>MNVASRVVVNADRVKGTINRNIYGHFSEHLGRCIYEGLWVGEDSPIPNTNGIRNDVLEALKQMKIPVLHWPGGCFADEYHWKDGVGPREKRKRMVNTHWGGVIENNHFGTHEFMMLCELLGCEPYISGNVGSGTVQEMSEWVEYITFDGESPMANWRRENGREKPWRIKYWGVGNENWGCGGNMRAEYYADLYRQFQTYLRNYGDNKLHKIACGAWTADYHWTEVLMKQAAPFMHGLSLHYYTVPGPWEKKGPATGFTTDEWWVTLKKALFMDELVTKHSAIMDVYDPDKRIDLIVDEWGTWYDVEPGTNPGFLYQQNSIRDALVAGATLHIFHRHCDRVRMANIAQLVNVMQSVILTEGERMLLTPTYHVFNMFKVHQDAELLDTWESVERTGPEGELPKVSVSASRAADGKIHISL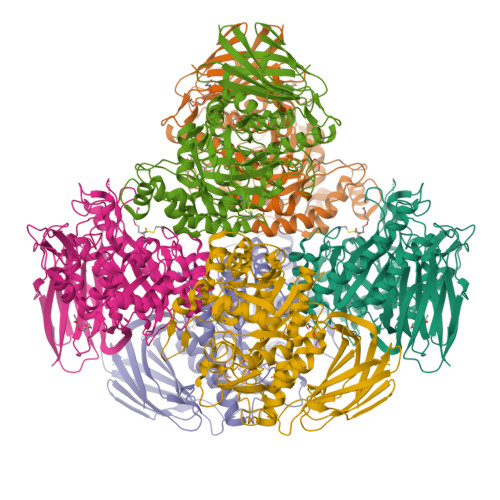CNLDFETGASVDIELRGLNGGVSATGTTLTSGRIDGHNTFDEPERVKPAPFRDFKLEGGHLNASLPPMSVTVLELTAG[3x]> GSHMSGIVPQLQNIVSTVNLGCKLDLKTIALRARNAEYNPKRFAAVIMRIREPRTTALIFSSGKMVCTGAKSEEQSRLAARKYARVVQKLGFPAKFLDFKIQNMVGSCDVKFPIRLEGLVLTHQQFSSYEPELFPGLIYRMIKPRIVLLIFV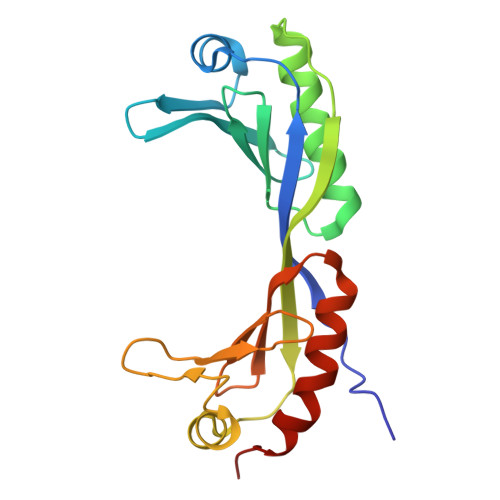SGKVVLTGAKVRAEIYEAFENIYPILKGFRKTT> MSNIEHGLSFIDIMVFAIYVAIIIGVGLWVSRDKKGTQKSTEDYFLAGKSLPWWAVGASLIAANISAEQ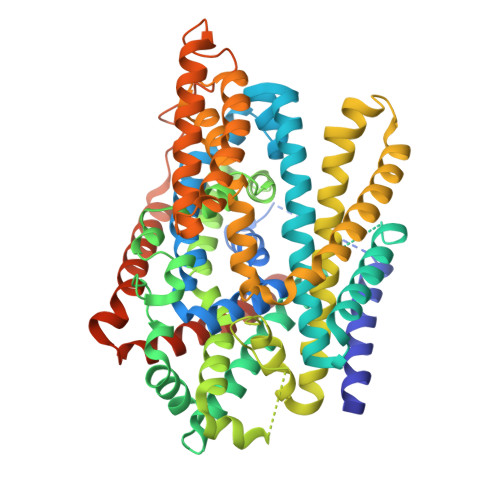FIGMSGSGYSIGLAIASYEWMSAITLIIVGKYFLPIFIEKGIYTIPEFVEKRFNKKLKTILAVFWISLYIFVNLTSVLYLGGLALETILGIPLMYSILGLALFALVYSIYGGLSAVVWTDVIQVFFLVLGGFMTTYMAVSFIGGTDGWFAGVSKMVDAAPGHFEMILDQSNPQYMNLPGIAVLIGGLWVANLYYWGFNQYIIQRTLAAKSVSEAQKGIVFAAFLALIVPFLVVLPGIAAYVITSDPQLMASLGDIAATNLPSAANADKAYPWLTQFLPVGVKGVVFAALAAAIVSSLASMLNSTATIFTMDIYKEYISPDSGDHKLVNVGRTAAVVALIIAALIAPMLGGIGQCFQYIQEYTGLVSPGILAVFLLGLFWKKTTSKGAIIGVVASIPFALFLKFMPLSMPFMDQMLYTLLFTMVVIAFTSLSTSINDDDPKGISVTSSMFVTDRSFNIAAYGIMIVLAVLYTLFWVNADAEITLIIFGVMAGVIGTILLISYGIKKLIKASYKSGGSPGHHHHHH>MDVVDPDIFNRDPRDHYDLLQRLGGGTYGEVFKARDKVSGDLVALKMVKMEPDDDVSTLQKEILILKTCRHANIVAYHGSYLWLQKLWICMEFCGAGSLQDIYQVTGSLSELQISYVCREVLQGLAYLHSQKKIHRDIKGANILINDAGEVRLADFGISAQIGAELARRLEFIGTPYWMAPEVAAVALKGGYNELCDIWSLGITAIELAELQPPLFDVHPLRVLFLMTKSGYQPPRLKEKGKWSAAFHNFIKVTLTKSPKKRPSATKMLSHQLVSQPGLNRGLILDLLDKLKNPGKGPSIGDI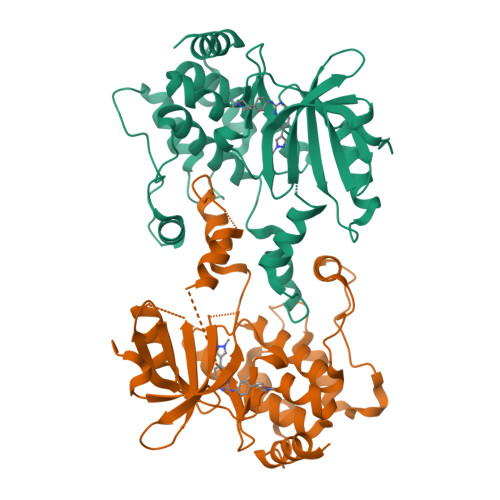EDEE[2x]>GSHMASMEMNKVLHQDLVQATRRILKLGPSELRVTDAGLICKNPNYSVCDAMLKTDTVYCVEYLLSYWESRTDHVPCFIFKNTGCAVSLCCFVRAPVKLVSPARHVGEFNVLKVNESLIVTLKDIEEIKPSAYGVLT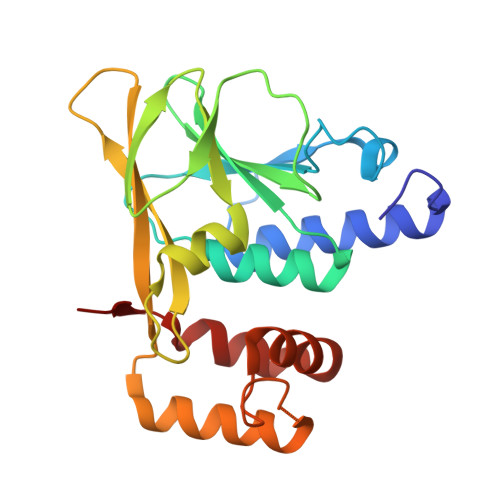KCVVRKSNSASVFNIELIAFGPENEGEYENLLRELYAKKAGGSGSGGSLTLHDLHDIFREHPELELKYLNMMKMAIT[2x]>SNAMTALETKADAEALINKEGIEYVSVRFTDLIGVQQHFTVPASEFLKDAFTDGMPFDGSSVEGFQAINESDMKLVPDVSTAFIDPFRKHKTLDVAFSIVDPLTDEPYSRDPRQVAGKAEAYLKSTGIADTASFAPEAEFFIFDKVRFENSMQRSFYEVDSIEAPWNSGIDTEDDGTPNIAFKNRVKKGYFPVPPIDHTQDLRDDMVANLQKVGLILERSHHEVAGAGQQEINYRFNSLQHAGDDLMKYKYVVHETAALAGKAATFMPKPIAGDNGTGMHCHQSLWKDGK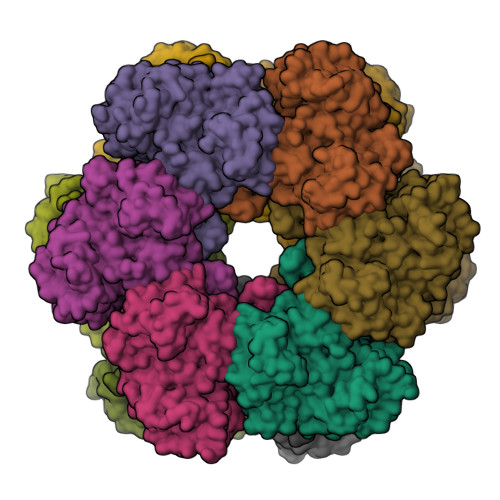PLFYDEKNYGGLSDLARWYIGGLIKHSSSVLAFTNPSLNSYHRLVPGFEAPVNLVYSARNRSAAIRIPLAGTSPAAKRIEFRAPDPSCNPFLAFSAQLMAGLDGILNHIEPPAPVDKDLYELPPEEHAGIKQVPSSLAEAMDALEEDHDFLTAGDVFTDDLIDTWISIKRGEIDQARLAPTPLEYELYFHI[6x]> MSTQYETQGYTINNAGRRLVVDPITRIEGHMRCEVNINDQNVITNAVSCGTMFRGLEIILQGRDPRDAWAFVERICGVCTGVHALASVYAIEDAIGIKVPDNANIIRNIMLATLWCHNHLVHFYQLAGMDWIDVLDALKADPRKTSELAQSLSSWPKSSPGYFFDVQNRLKKFVEGGQLGIFRNGYWGHPQYKLPPEANLMGFAHYLEALDFQREIVKIHAVFGGKNPHPNWIVGGMPCAINIDESGAVGAVNMERLNLVQSIITRTADFINNVMIPDALAIGQFNKPWSEIGTGLSDKCVLSYGAFPDIANDFGEKSLLMPGGAVINGDFNNVLPVDLVDPQQVQEFVDHAWYRYPNDQVGRHPFDGITDPWYNPGDVKGSDTNIQQLNEQERYSWIKAPRWRGNAMEVGPLARTLIAYHKGDAATVESVDRMMSALNLPLSGIQSTLGRILCRAHEAQWAAGKLQYFFDKLMTNLKNGNLATASTEKWEPATWPTECRGVGFTEAPRGALGHWAAIRDGKIDLYQCVVPTTWNASPRDPKGQIGAYEAALMNTKMAIPEQPLEILRTLHSFNPCLACS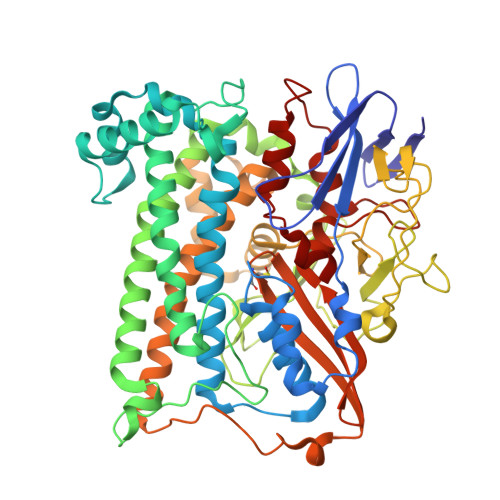TH>[2x]HMLNVGATAPDFTLRDQNQQLVTLRGYRGAKNVLLVFFPLAFTGICQGELDQLRDHLPEFENDDSAALAI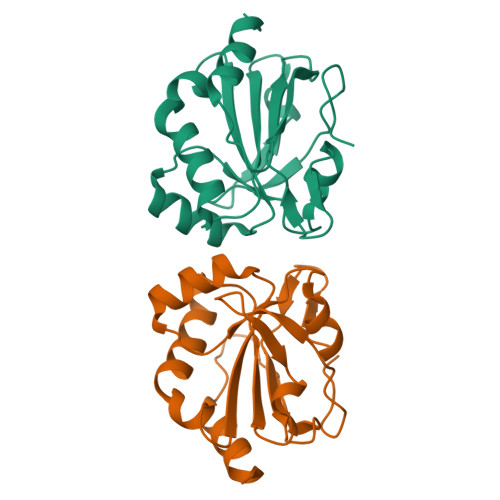SVGPPPTHKIWATQSGFTFPLLSDFWPHGAVSQAYGVFNEQAGIANAGTFVVDRSGIIRFAEMKQPGEVRDQRLWTDALAALT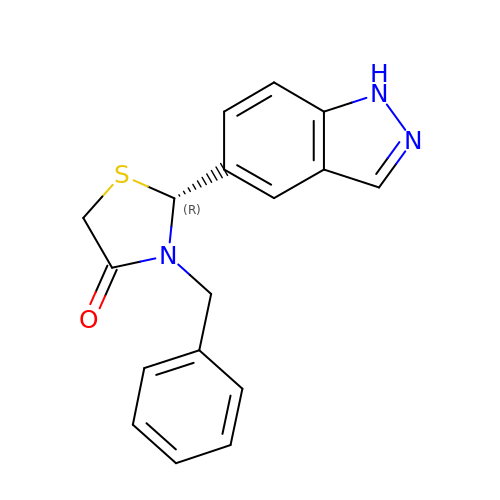(2R)-3-benzyl-2-(1H-indazol-5-yl)-1,3-thiazolidin-4-one | C17 H15 N3 O S | UIFSOMZAJQOGHJ-QGZVFWFLSA-N>MSEYIRVTEDENDEPIEIPSEDDGTVLLSTVTAQFPGACGLRYRNPVSQCMRGVRLVEGILHAPDAGWGNLVYVVNYPKDNKRKMDETDASSAVKVKRAVQKTSDLIVLGLPWKTTEQDLKEYFSTFGEVLMVQVKKDLKTGHSKGFGFVRFTEYETQVKVMSQRHMIDGRWCDCKLPNSKQSQDEPLRSRKVFVGRCTEDMTEDELREFFSQYGDVMDVFIPKPFRAFAFVTFADDQIAQSLCGEDLIIKGISVHISNAEPKHNSNRQLERSGRFGGNPGGFGNQGGFGNSRGGGAGLGNNQGSNMGGGMNFGAFSINPAMMAAAQAALQSSW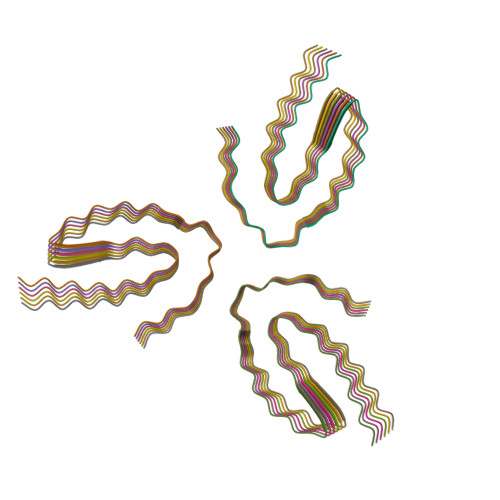GMMGMLASQQNQSGPSGNNQNQGNMQREPNQAFGSGNNSYSGSNSGAAIGWGSASNAGSGSGFNGGFGSSMDSKSSGWGM[18x]N-[(1R)-1-(2,4-dichlorophenyl)-2-(1H-imidazol-1-yl)ethyl]-4-(5-phenyl-1,3,4-oxadiazol-2-yl)benzamide 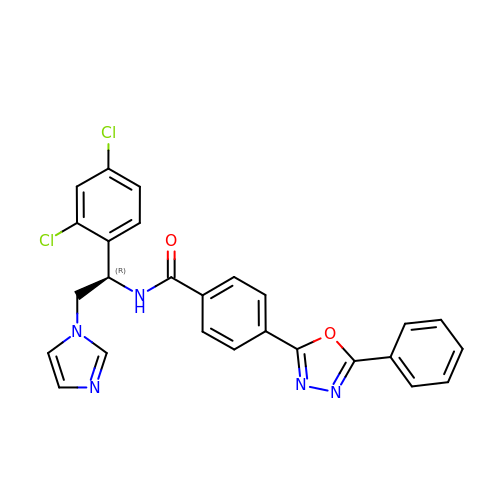| C26 H19 Cl2 N5 O2 | CJPLMXOWZZCYHJ-QHCPKHFHSA-N>GSDELYRQSLEIISRYLREQATGAKDTKPMGRSGATSRKALETLRRVGDGVQRNHETAFQGMLRKLDIKNEDDVKSLSRVMIHVFSDGVTNWGRIVTLISFGAFVAKHLKTINQESCIEPLAESITDVLVRTKRDWLVKQRGWDGFVEFFHVEDLEGG[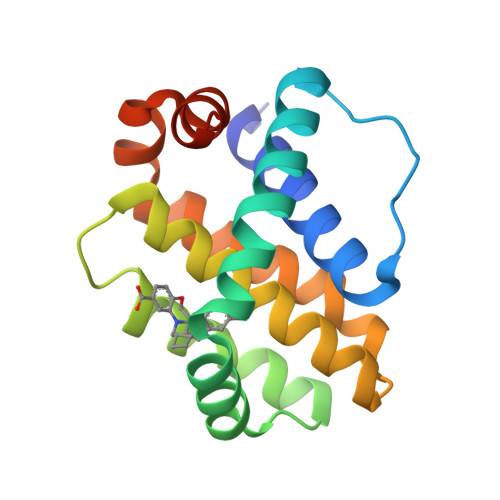2x]> GSHMAKHEQILVLDPPSDLKFKGPFTDVVTTNLKLQNPSDRKVC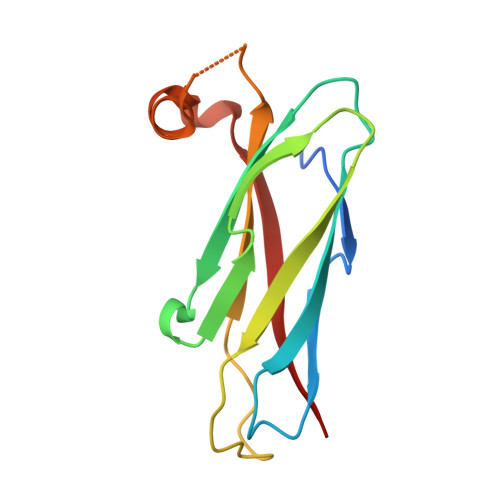FKVKTTAPRRYCVRPNSGVIDPGSIVTVSVMLQPFDYDPNEKSKHKFMVQTIFAPPNISDMEAVWKEAKPDELMDSKLRCVFEM> PELPEVETVRRELEKRIVGQKIISIEATYPRMVLTGFEQLKKELTGKTIQGISRRGKYLIFEIGDDFRLISHLRMEGKYRLATLDAPREKHDHLTMKFADGQLI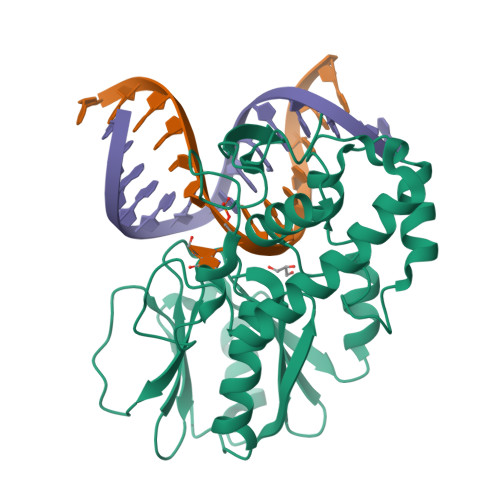YADVRKFGTWELISTDQVLPYFLKKKIGPEPTYEDFDEKLFREKLRKSTKKIKPYLLEQTLVAGLGNIYVDEVLWLAKIHPEKETNQLIESSIHLLHDSIIEILQKAIKLGGSSIRTYSALPSTGKMQNELQVYGKTGEKCSRCGAEIQKIKVAGRGTHFCPVCQQK PINACOL[[2-AMINO-ALPHA-(1-CARBOXY-1-METHYLETHOXYIMINO)-4-THIAZOLEACETYL]AMINO]METHANEBORONATE 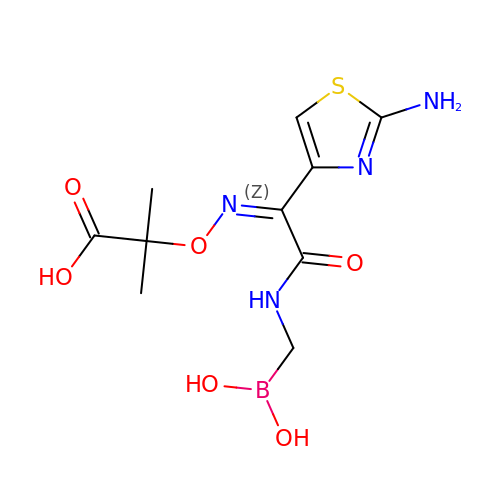| C10 H15 B N4 O6 S | ZECCQELUYUPTSB-UUASQNMZSA-N>UAAGUUCUCGAUCUUUAAAAUCGUUAGCUCGCCAGUUAGCGAGGUCUGCGAAAGCAGAUAAUCGGGUGCAACUCCCGCCCUUUCUCCGAGGGUCAUCGGAACCA[2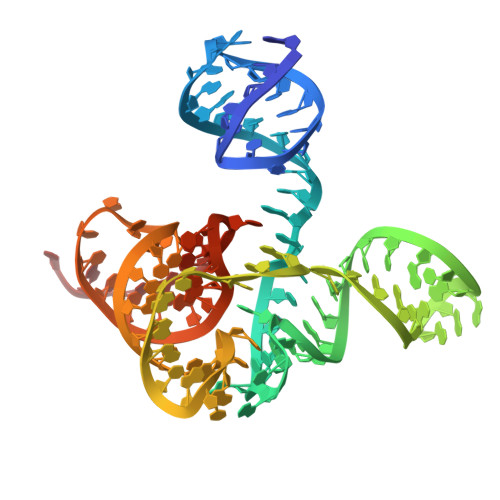x]>PSVYDAAAQLTADVKKDLRDSWKVIGSDKKGNGVALMTTLFADNQETIGYFKRLGDVSQGMANDKLRGHSITLMYALQAFIDQLDNPDDLVCVVEKFAVNHITRKISAAEFGKINGPIKKVLASKNFGDK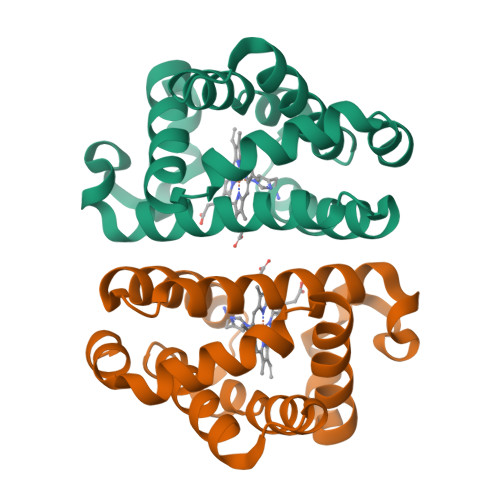YANAWAKLVAVVQAAL[2x]>[3x]MTPASYNLAVRRAAPAVVNVYNRGLNTNSHNQLEIRTL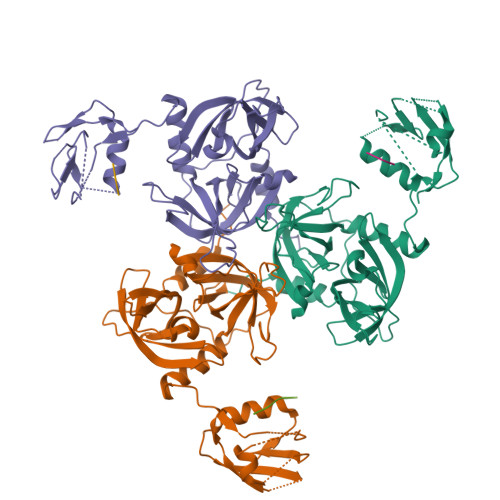GSGVIMDQRGYIITNKHVINDADQIIVALQDGRVFEALLVGSDSLTDLAVLKINATGGLPTIPINARRVPHIGDVVLAIGNPYNLGQTITQGIISATGRIGLNPTGRQNFLQTDASINHGNSGGALVNSLGELMGINTLSFDKSNDGETPEGIGFAIPFQLATKIMDKLIRDGRVIRGYIGIGGREIAPLHAQGGGIDQLQGIVVNEVSPDGPAANAGIQVNDLIISVDNKPAISALETMDQVAEIRPGSVIPVVVMRDDKQLTLQVTIQEYPATN;>DNRLGLVYQF[3x]4-IODO-ACETAMIDO 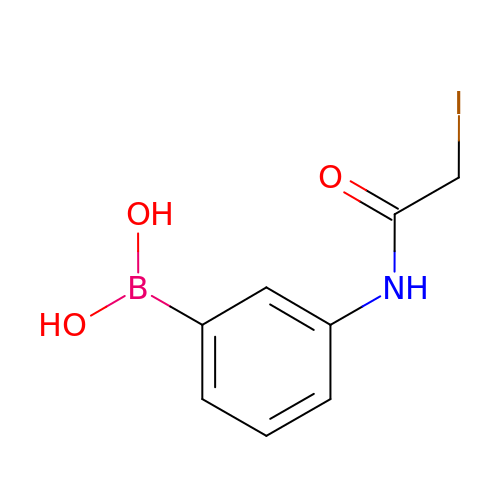PHENYLBORONIC ACID | C8 H9 B I N O3 | LMHXPDZPXBIIEX-UHFFFAOYSA-N3-(2-pyrimidin-4-ylethyl)-1~{H}-indole | C14 H13 N3 | 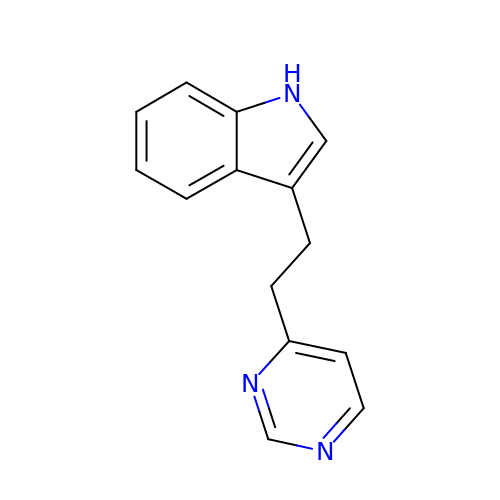VEEXILNZSSXTHF-UHFFFAOYSA-N> IKGNQKKQKGKNQSNNNNNIREEGKQIKEMILPHNNRQLARQYFDSLPENDINRKYYEGLKYETPKTFFGRFLNQFNIDAKLDTLSKFYTYQKTIRATQAELQ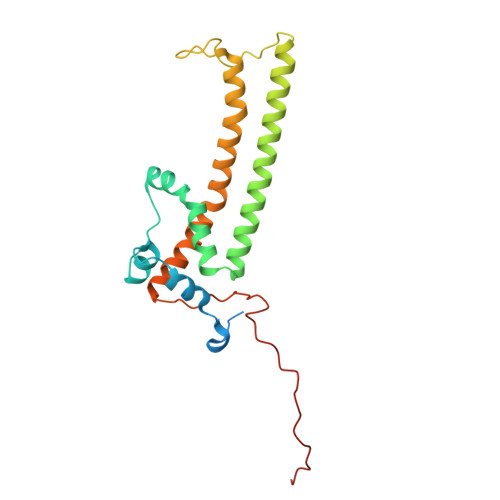EDRKSYLTNSLLFTAVSWFSIYQFARKGAVLPVLREYGRYFGTHRLFRQYLHTLVLPLLYTEYALNQKYYTHMEHLWTVHVNRLNQKILEDPLYTFYPQELNVPKHNIIVPTIFRDTPQ>MSRAKVGINGFGRIGRLVLRAAFLKNTVDVVSVNDPFIDLEYMVYMIKRDSTHGTFPGEVSTENGKLKVNGKLISVHCERDPANIPWDKDGAEYVVESTGVFTTIDKAQAHIKNNRAKKVIISAPSADAPMFVVGVNENSYEKSMSVVSNASCTTNCLAPLAKVIHDKFEIVEGLMTTVHSFTATQKVVDGPSSKLWRDGRGAMQNIIPASTGAAKAVGKVIPALNGKLTGMAFRVPTPDVSVVDLTCRLGKGASYEEIKAAVKAAASGPLKGILEYTEDEVVSSDFVGSTSSSI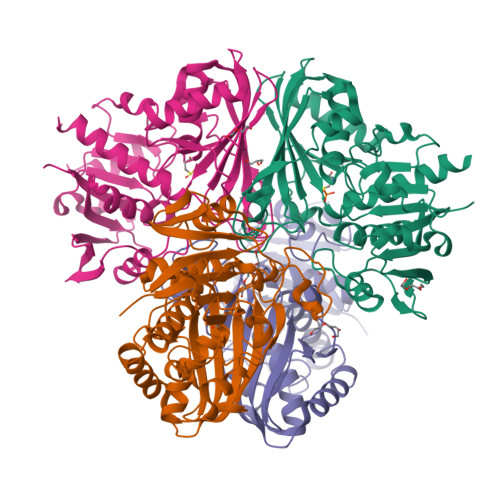FDAKAGISLNNNFVKLVSWYDNEFGYSCRVVDLITHMHKVDHA[4x]>ETAGVVTGKTLPITKSMIYTDNEILMPKTTFTFTIEPDTTASGKTKDGLEIKSGETTGLTTKAIVSYDNTDKESAKNKTSNFNFETVTFSGIGIYRYTVSEQNDGIEGIQYDGKKWTVDVYVGNKEGGGFEPKYVVSKEVNSDVKKPIRFENSFKTTSLKIEKQVTGNTGELQKDFNFTLILEASALYEKGQVVKIIQDGQTKDVVIGQEYKFTLHDHQSIMLAKLPIGISYKLTEDKADGYTTTATLKEGEIDAK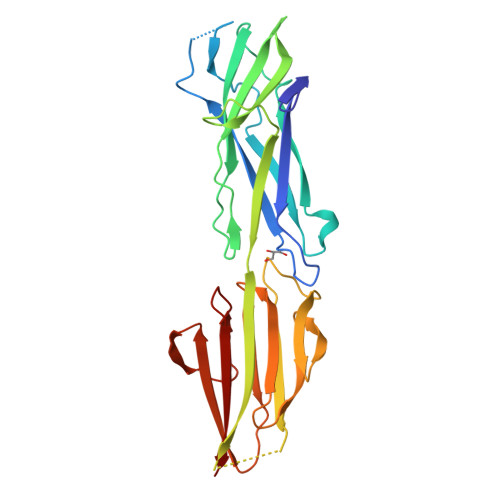EYVLGNLQKTDESADEIVVTNKRD[2x]Here, we have investigated the structure and function of a Mtb methyltransferase (MTase) Rv2067c. It secretes methyltransferase (MTase) Rv2067c into macrophages, trimethylating histone H3K79 in a non-nucleosomal context. Rv2067c downregulates host MTase DOT1L, decreasing DOT1L-mediated nucleosomally added H3K79me3 mark on pro-inflammatory response genes. We provide the structural basis for how Rv2067c methylates free histone H3 and not nucleosomal H3 by comparing its structure with that of the nucleosome-bound DOT1L, which catalyzes H3K79 methylation only in the nucleosomal context.

To understand the structural differences conferring the context-dependent methylation of H3K79 by DOT1L and Rv2067c, and the basis of free H3 methylation by Rv2067c, we determined the structure of Rv2067c to 2.40 Å resolution. Each monomer (407 aa) of Rv2067c homodimer (Source Data and Supplementary Software File 1) is composed of three domains: N-terminal SAM-binding catalytic domain (CD), dimerization domain (DD), and C-terminal domain (CTD). The catalytic domain contains a central seven-stranded β-sheet flanked by α-helices, a characteristic of seven-β-strand (7BS) MTases (class-I MTases)35. The DD is composed of two subdomains separated on the primary structure, namely the large subdomain (LSD; residues 163-230, four α-helices) and the small subdomain (SSD; residues 257-291, two α-helices), which are inserted into the catalytic domain at β5-α5 and β6-β7 loops, respectively. Dimer is formed by the cross-subdomain interactions between the DDs of the two monomers A and B in a fashion: LSDA-SSDB and LSDB-SSDA, and LSDA-LSDB. CTD is about 100 residues long with α + β architecture. The dimerization interface, in conjunction with the other two domains, forms two parallel trough-like structures across the dimer, which constitute the acceptor substrate-binding trough. The active site lies at one end of the trough, deep inside the protein, encompassed by CD and LSD. Inspection of the Rv2067c substrate-binding trough revealed that the residues facing the methyl moiety of SAM (SAM-facing residues) occlude the H3K79 binding. In addition to the active site dynamics, the dα3-dα4 loop (residues 209–214, part of LSD and the substrate-binding trough) near the active site is disordered, as evident from the missing electron density in the crystal structure and relatively high root mean square fluctuations observed from simulations (Source Data and Supplementary Software File 3). In short, due to the lack of nucleosome interacting structural appendages and different active site architecture, Rv2067c is incompetent to methylate nucleosomal H3K79, but its substrate-binding trough could accomodate free H3 for methylation.

>[2x]GAMVTDDHPRADIVSRQYHRWLYPHPIADLEAWTTANWEWFDPVHSHRILWPDREYRPDLDILIAGCGTNQAAIFAFTNRAAKVVAIDISRPALDHQQYLKDKHGLANLELHLLPIEELATLGRDFDLVVSTGVLHHLADPRAGMKELAHCLRRDGVVAAMLYGKYGRIGVELLGSVFRDLGLGQDDASIKLAKEAISLLPTYHPLRNYLTKARDLLSDSALVDTFLHGRQRSYTVEECVDLVTSAGLVFQGWFHKAPYYPHDFFVPNSEFYAAVNTLPEVKAWSVMERLETLNATHLFMACRRDRPKEQYTIDFSTVAALDYVPLMRTRCGVSGTDMFWPGWRMAPSPAQLAFLQQVDGRRTIREIAGCVARTGEPSGGSLADLEEFGRKLFQSLWRLDFVAVALPASG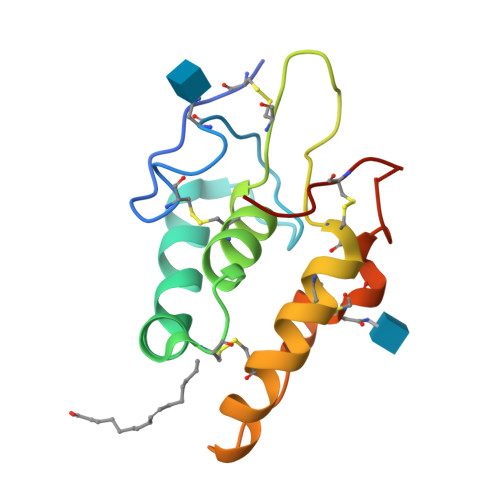>EEERRCDPIRISMCQNLGYNVTKMPNLVGHELQTDAELQLTTFTPLIQYGCSSQLQFFLCSVYVPMCTEKINIPIGPCGGMCLSVKRRCEPVLKEFGFAWPESLNCSKFPPQNDHNHMCMEGPGD[2x]> NPVENYIDEVLNEVLVVPNINSSNPTTSNSAPALDAAETGHTSSVQPEDVIETRYVQTSQTRDEMSLESFLGRSGCIHESKLEVTLANYNKENFTVWAINLQEMAQIRRKFELFTYTRFDSEITLVPCISALSQDIGHITMQYMYVPPGAPVPNSRDDYAWQSGTNASVFWQHGQAYPRFSLPFLSVASAYYMFYDGYDEQDQNYGTANTNNMGSLCSRIVTEKHIHKVHIMTRIYHKAKHVKAWCPRPPRALEYTRAHRTNFKIEDRSIQTAIVTRPIITTAGPSDMY;> SPTVEACGYSDRIIQITRGDSTITSQDVANAIVAYGVWPHYLSSKDASAIDKPSQPDTSSNRFYTLRSVTWSSSSKGWWWKLPDALKDMGIFGE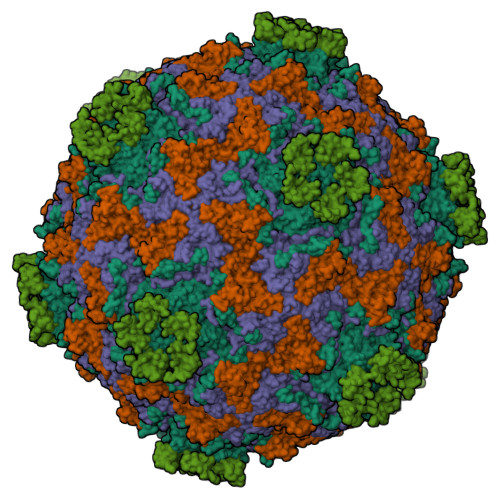NMFYHYLGRSGYTIHVQCNASKFHQGTLIVALIPEHQIASALHGNVNVGYNYTHPGETGREVKAETRLNPDLQPTEEYWLNFDGTLLGNITIFPHQFINLRSNNSATIIAPYVNAVPMDSMRSHNNWSLVIIPICPLETSSAINTIPITISISPMCAEFSGARAKRQ;> GLPVFITPGSGQFLTTDDFQSPCALPWYHPTKEISIPGEVKNLVEICQVDSLVPINNTDTYINSENMYSVVLQSSINAPDKIFSIRTDVASQPLATTLIGEISSYFTHWTGSLRFSFMFCGTANTTVKLLLAYTPPGIAEPTTRKDAMLGTHVIWDVGLQSTISMVVPWISASHYRNTSPGRSTSGYITCWYQTRLVIPPQTPPTARLLCFVSGCKDFCLRMARDTNLHLQSGAIAQ;> GAQVSRQNVGTHSTQNSVSNGSSLNYFNINYFKDAASNGASKLEFTQDPSKFTDPVKDVLEKGIPTLQ;> CRIHEISCGAHSTQCIPVSWRCDGENDCDSGEDEENCGN2-methylsulfonyl-N-(1-methyl-1,2,3,4-tetrazol-5-yl)-4-(trifluoromethyl)benzamide | C11 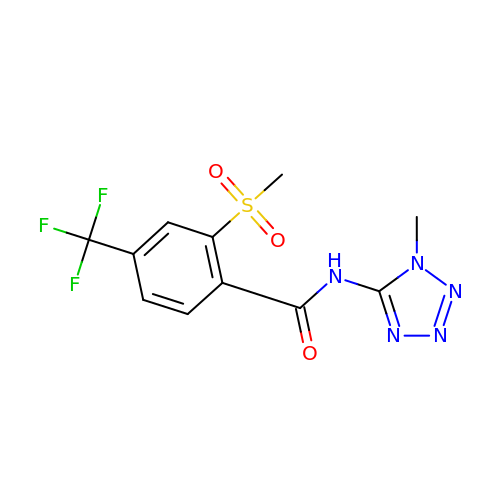H10 F3 N5 O3 S | XOZLZZGMRLKTTP-UHFFFAOYSA-N> MSKKQPKPVKAEQLKSYYEESRGLERDLIGEFVKSRKTAWRVATASGLFGLLGMVCGIVGFSQPAPAPLVLRVDNATGAVDVVTTLREHESSYGEVVDTYWLNQYVLNREAYDYNTIQMNYDTTALLSAPAVQQDYYKLFDGSNARDRVLGNKARITVRVRSIQPNGRGQATVRFTTQQHNSNGTVEAPQHQIATIGYTYIGAPMRSSDRL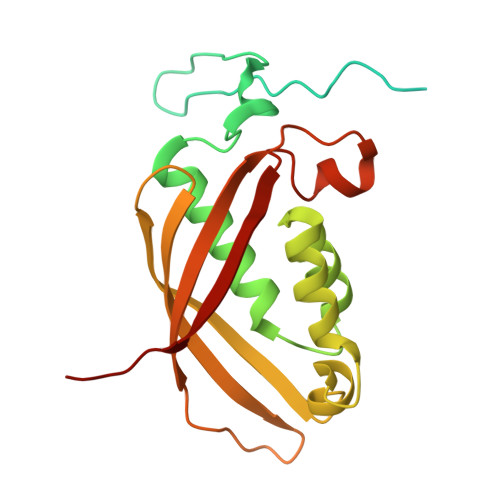LNPLGFQVTSYRADPEILNN>[3x]GPLGSMSEFRIHHDVNELISLLHVFGLEGADVYIDLLQKNRTPYVTTSVSTHSAKVKIAEFSRTPDDFLKKYEELKSKNTRNLDPLVYLLSKLIEDKETLQYLQQNAKDKAELAT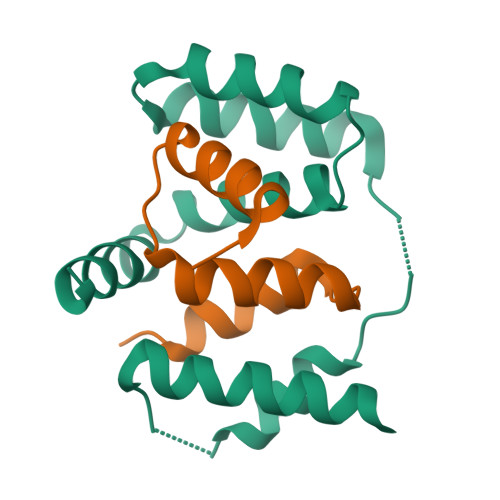SSVTSVSLPIAPNTSKISMQELEELRRQLETATVAVSCSHQPVEVLRKFLRDK;>GPHMMSRGQTEGSQAMASSQAAGPGPSPDAIVSVSGTVQKYVAKKKKVLNPEEAELYELTQAAGIVIDQEVFKILVDLLKMNVAPLAVFQMLKSMCAG[3x]> MATQAKRPRVAGPVDGGDLDPVACFLSWCRRVGLELSPKVAVSRQGTVAGYGMVARESVQAGELLFVVPRAALLSQHTCSIGGLLERERVALQSQSGWVPLLLALLHELQAPASRWRPYFALWPELGRLEHPMFWPEEERRCLLQGTGVPEAVEKDLANIRSEYQSIVLPFMEAHPDLFSLRVRSLELYHQLVALVMAYSFQEPLEEEEDEKEPNSPVMVPAADILNHLANHNANLEYSANCLRMVATQPIPKGHEIFNTYGQMANWQLIHMYGFVEPYPDNTD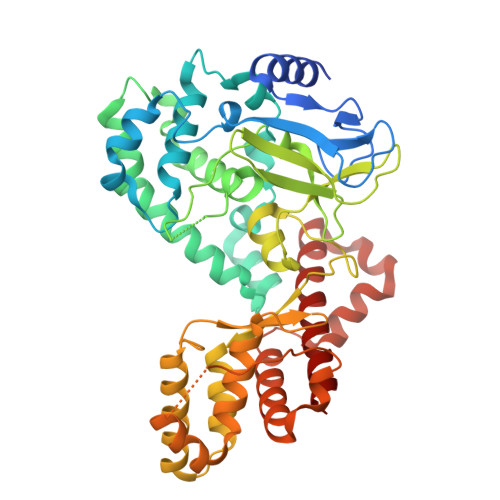DTADIQMVTVREAALQGTKTEAERHLVYERWDFLCKLEMVGEEGAFVIGREEVLTEEELTTTLKVLCMPAEEFRELKDQDGGGDDKREEGSLTITNIPKLKASWRQLLQNSVLLTLQTYATDLKTDQGLLSNKEVYAKLSWREQQALQVRYGQKMILHQLLELTS> MSKAKIGIVTVSDRASAGITADISGKAIILALNLYLTSEWEPIYQVIPDEQKVI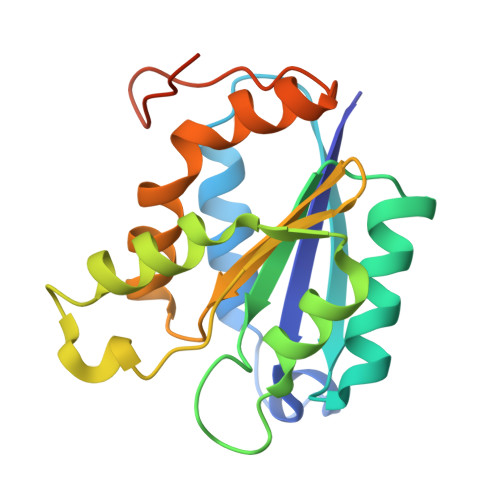ETTLVKMADIQDCCLIVTTGGTGPAKRDVTPEATEAVCDRMMPGFGELMRAESLKEVPTAILSRQTAGLRGDSLIVNLPGDPASISDCLLAVFPAIPYCIDLMEGPYLECNEAMIKPFRPKAKLEHHHHHH> ACLNTRFLEEE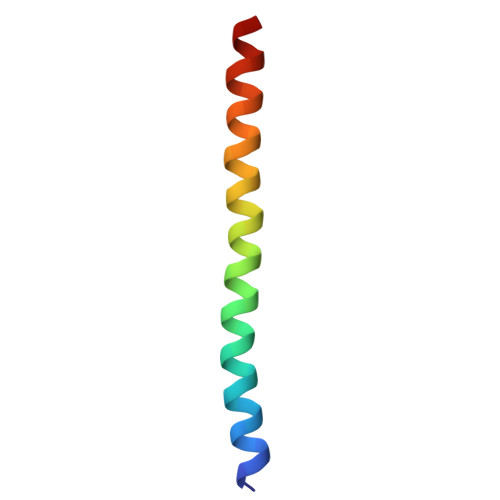ELRSHHILERLDAHIEELKRESEKTVRQFTALK Supporting this hypothesis, we here determined the fibril structure of two AMPs from amphibians, uperin 3.5 and aurein 3.3, by cryogenic electron microscopy (cryo-EM), revealing amyloid cross-β fibrils of mated β-sheets at atomic resolution. For both of the studied ffAMPs, cryo-EM data unambiguously prove an amyloid cross-β structure comprised of β-sheets with tightly coupled dry interfaces and strands perpendicular to the fibril axis. Despite the dissimilarity in lateral fibril structure and the difference of extended versus kinked β-sheets, the 17-residue ffAMPs uperin 3.5 and aurein 3.3 are remarkably similar in their residue composition. Overall, compared to other amyloids, the sequence content of the two AMPs indicates a dominant apolar and positively charged nature, which fits the functional interactions with negatively charged bacterial membranes.

The cross-α form was also recently shown by the crystal structure of the antibacterial peptide uperin 3.5 secreted by Uperoleia mjobergii (Mjoberg’s toadlet), which forms fibrils with amyloid properties. Here, a cryo-EM study of uperin 3.5 in the absence of lipids reveals the presence of β-rich fibril polymorphs, and the atomic details of the cross-β configuration, allowing for a direct comparison to the cross-α fibril and exposing the substantial polymorphism of the same sequence. While the unique morphology of the most abundant polymorph (type I; relative abundance 71%) makes both individual fibrils in the micrographs and two-dimensional class averages easy to identify, variations between the other fibril types are more subtle. We find a propeller-shaped structure with threefold rotational symmetry about the fibril axis, where each of the three asymmetric units per filament layer comprises three chains (labeled A, B, C, along with their symmetry equivalents: A’, A”, etc.) of distinct conformation. An atomic model of the uperin 3.5 peptide built into each asymmetric unit (propeller blades) shows excellent agreement with the data in the inner section of the fibrils, comprising full-length (17 residues) monomers in chain A, and 14 and 7 residues in chains B and C, respectively. Chains A and B are tightly interdigitated and form β-sheets along the fibril axis, both hallmark features of a canonical amyloid cross-β fibril. Chain C is almost perpendicular to the other two. The center of the uperin 3.5 propeller is composed of inward-facing Arg7 and Leu5 residues from chains A, A’ and A”, creating a positively charged and hydrophobic core. In the cross-β fibril, Arg7 on chains A, A’ and A” is buried in the core of the fibril, while on chains B, B’ and B”, it is facing outwards, but with the charge being compensated by interactions with Asp4. Inaccessible charge of Arg7 in the cross-β fibril might support an inactive storage form in contrast to interacting with bacterial membranes.

>GVGDLIRKAVSVIKNIVX[27x]>MVKTVAVMVGSLRKDSLNHKLMKVLQKLAEGRLEFHLLHIGDLPHYNDDLWADAPESVLRLKDRIEHSDAVLAITPEYNRSYPGMIKNAIDWATRPYGQ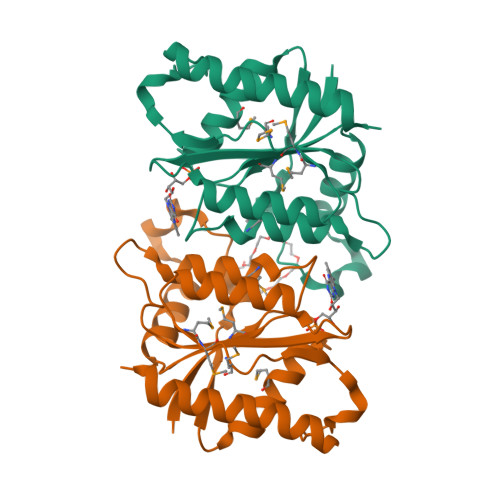NSWKGKPAAVIGTSPGVIGAALAQARLKNDLLHVGTVMMSMPEAYIQWHAEAYAADGSVTDEKTAKFLQGFVDAFVDWIEKHGLEHHHHHH[2x]Here we characterize a metal-dependent, bifunctional isoprenyl diphosphate synthase from the leaf beetle Phaedon cochleariae by structural and functional analyses. Isoprenyl diphosphate synthase in P. cochleariae (PcIDS1, EC 2.5.1.1) produces FPP in the presence of Mg2+, but preferably forms GPP when exposed to the heavy metal ions (HMIs) Co2+ or Mn2+. Inter- and intramolecular cooperative effects in the homodimer strongly depend on the provided metal ions and regulate the biosynthetic flux of terpene precursors to either biological defence or physiological development. Strikingly, a unique chain length determination domain adapts to form geranyl or farnesyl pyrophosphate by altering enzyme symmetry and ligand affinity between both subunits.

Stabilized by cation–π interactions with R427, the F315 side chain positions IPPHAl for nucleophilic attack. V286 and I420 form the bottom of this specificity pocket and act as a molecular ruler, whereas F282 and F315 engage in π-stacking with both allyl groups.

>[2x]GSFSKEESREFMAIFPDIVRDLTDAGRHTDIPEVTKRFAKVLQYNVPTGKKTRGLSTVIAYKMLEKPENLTPENVRLAGILGWCVELLQASLLIMDDLMDRSETRRGQPCWYRQENVGFLAINDCLHVESSLYSVLRKYFSHLPCYVPIIELFHDVNFKTNMGQSLDALCMKDGRPILSQFTMKRYSSIVKYKTSYYTFQLPVSLGMYLADMYDPEQHRQAKTILMEIGEFAQIQDDFLDAFGDSQVTGKVGTDIKEGKCSWLAVVALQRSNPAQRQIMEEHYGRPEPESTQIIKNLYIELGLPATFAVYEEESFNIIRTHIHQISKGLPHDLFFKIMKKIYKRDA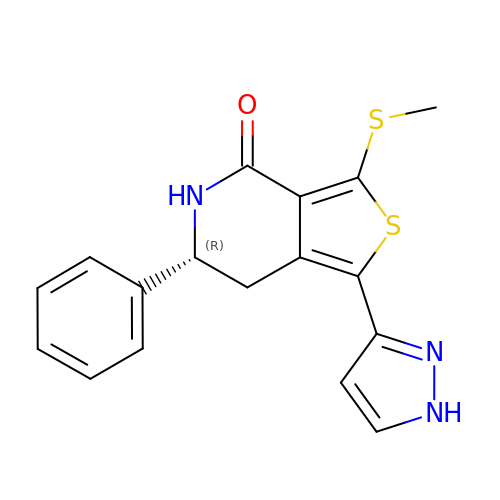(6R)-3-(methylsulfanyl)-6-phenyl-1-(1H-pyrazol-3-yl)-6,7-dihydrothieno[3,4-c]pyridin-4(5H)-one | C17 H15 N3 O S2 | JFNXRABTLWJEOU-CYBMUJFWSA-N>GSAAASSVDTSQEFQNNLKNAIGNLPFQYVNGIYELNNNQTNLNADVNVKAYVQNTIDNQQRPSTANAMLDRTIRQYQNRRDTTLPDANWKPLGWHQVATNDHYGHAVDKGALIAYALAGNFKGWDASVSNPQNVVTQTAHSNQSNQKINRGQNYYESLVRKAVDQNKRVRYRVTPLYRNDTDLVPFAMHLEAKSQDGTLEFNVAIPNTQASYTMDYATGEITLN[2x]

One such nuclease, NucA (Gbs0661) from S. agalactiae (henceforth referred to as GBS_NucA), has been shown to degrade NETs and to improve infection persistence in the host. GBS_NucA is thought to be a sequence-nonspecific DNA/RNA nuclease with endonucleolytic and exonucleolytic activity. Although this family of nucleases share a common ββα metal-finger catalytic core and reaction mechanism, their global structures, localization and regulatory mechanisms can vary widely. As a starting point for such development, we have determined high-resolution X-ray crystal structures of GBS_NucA with and without bound magnesium ion and compared them with those of other ββα metal-finger nucleases.

Because wild-type GBS_NucA is difficult to overexpress in E. coli, an inactive form of the enzyme, H148A, was used. A 1.5 Å high-resolution X-ray crystal structure of the GBS_NucA (H148A) apoprotein was obtained in space group P1 in the absence of a divalent metal. Two molecules of GBS_NucA were present in the asymmetric unit. Because the crystallization conditions lacked divalent metal ions, the active site was solvated but otherwise empty. An intricate network of putative hydrogen-bonding interactions links the metal in the active center through Asn179 to the distally located Gln180 and His142, using Asp145 as the intermediary. This network is also present in the apoprotein, where the metal-binding site is unoccupied. Given that this coil is entirely disordered in the P1 crystal form and is incomplete in molecules C and D of the P63 crystal form, we hypothesize that it is highly mobile in the absence of a DNA substrate. Residues Arg116–Asp118 along this loop form a short α-helix (henceforth referred to as α-helix S), although there are no such indications of helical propensity in Arg116–Asp118 in the P1 crystal form. The ββα motif is comprised of β-strands 7 and 8, the latter of which connects directly to α-helix C. The compact active site is outlined by this motif and its deepest recess is formed by the core β-sheet (β-strands 4, 9 and 10).> APEITEEMEKEIKNVFRNGNQDEVLSEAFRLTIT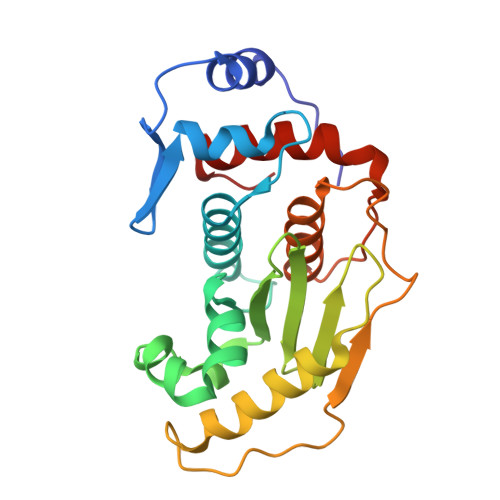RKDIQTLNHLNWLNDEIINFYMNMLMERSKEKGLPSVHAFNTFFFTKLKTAGYQAVKRWTKKVDVFSVDILLVPIHLGVHWCLAVVDFRKKNITYYDSMGGINNEACRILLQYLKQESIDKKRKEFDTNGWQLFSKKSQIPQQMNGSDCGMFACKYADCITKDRPINFTQQHMPYFRKRMVWEILHRKLL>MHHHHHHSSGRENLYFQGMPLRLDIKRKLTARSDRVKSVDLHPTEPWMLASLYNGSVCVWNHETQTLVKTFEVCDLPVRAAKFVARKNWVVTGADDMQIRVFNYNTLERVHMFEAHSDYIRCIAVHPTQPFILTSSDDMLIKLWDWDKKWSCSQVFEGHTHYVMQIVINPKDNNQFASASLDRTIKVWQLGSSSPNFTLEGHEKGVNCIDYYSGGDKPYLISGADDRLVKIWDYQNKTCVQTLEGHAQNVSCASFHPELPIIITGSEDGT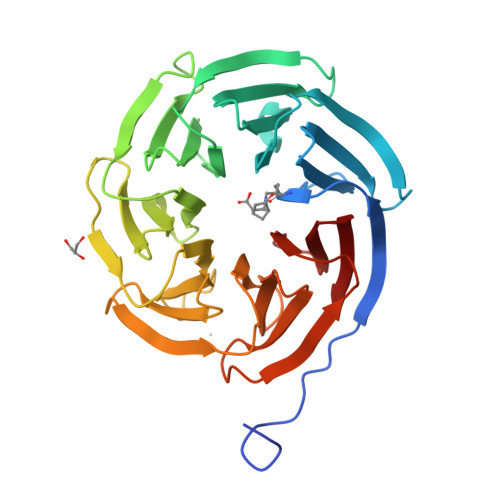VRIWHSSTYRLESTLNYGMERVWCVASLRGSNNVALGYDEGSIIVKLG[2x]Replication Protein A (RPA) is an abundant multi-domain heterotrimeric protein complex essential to nearly all DNA processing events inside eukaryotic cells. RPA is thus a critical component for replication, repair, and recombination pathways. The largest subunit, Rfa1, possesses four OB domains: DNA-binding domain-A (DBD-A), B (DBD-B), C (DBD-C), and F (DBD-F), which are connected by flexible linkers. The smallest subunit Rfa3 has a single OB-fold (DBD-E) and forms part of the trimerisation core (Tri-C) consisting of DBD-C of Rfa1, DBD-D of Rfa2, and DBD-E of Rfa3.

We produced recombinant full-length S. cerevisiae RPA heterotrimer complexes of Rfa1, Rfa2, and Rfa3 in bacteria (denoted as ScRPA). Recombinant ScRPA was purified to homogeneity as judged by SDS–PAGE and gel filtration analysis coupled with in-line multi-angle laser light scattering (SEC-MALS), suggesting intact complexes. We used a 100 nt polypyrimidine oligonucleotide to form a RPA-ssDNA complex containing multiple RPA molecules (dT100 and Supplementary Fig. 2a, b). Combining two datasets and several rounds of 2D and 3D classification we isolated a fraction of the particles that enabled a 3D reconstruction corresponding to the ScRPA Tri-C associated with ssDNA to a global resolution of 4.7 Å, a surprisingly high-resolution structure by cryoEM given the small size of the protein–nucleic acid complex (~55 kDa with ssDNA). Although full-length proteins were used to form the ScRPA-ssDNA complexes,, the winged-helix domain, as well as some of the N-terminus of Rfa2 were invisible. The reconstruction measures ~81 Å × ~58 Å × ~36 Å in dimensions and a model of the ScRPA Tri-C (based on homology models) can be fitted into the EM density map. Subsequently, the model was flexibly fitted using molecular dynamics flexible fitting (MDFF)32,33 and further refined using jelly-body refinement routines in Refmac534 within CCPEM35, and real-space refinement procedures in Phenix36. There are a number of yeast-specific insertions compared to the human or fungal structures, the most obvious being for DBD-D and DBD-E. The presence of ssDNA in the reconstruction is further supported by the observation that in the absence of ssDNA, RPA molecules do not assemble into dimers and trimers and the majority of the Tri-C particles were isolated from dimers and trimers. We were able to reconstruct the relatively small Tri-C stably bound to a 20-nt segment of the ssDNA to surprisingly high resolution given its low molecular mass (~55 kDa). Our studies suggest that DBD-A/DBD-B may be more dynamic than previously thought, whereas the trimerization core is more stable on ssDNA.

> MASETPRVDPTEISNVNAPVFRIIAQIKSQPTESQLILQSPTISSKNGSEVEMITLNNIRVSMNKTFEIDSWYEFVCRNNDDGELGFLILDAVLCKFKENEDLSLNGVVALQRLCKKYPEIY;> TNTRVNTLTPVTIKQILESKQDIQDGPFVSHNQELHHVCFVGVVRNITDHTANIFLTIEDGTGQIEVRKWSEDAAQQFEIGGYVKVFGALKEFGGKKNIQYAVIKPIDSFNEVLTHHLEVIKCHSIASGMMK;> KFIAQRITIARAQAENLGRSEKGDFFSVKAAISFLKVDNFAYPACSNENCNKKVLEQPDGTWRCEKCDTNNARPNWRYILTISIIDETNQLWLTLFDDQAKQLLGVDANTLMSLKEEDPNEFTKITQSIQMNEYDFRIRAREDTYNDQSRIRYTVANLHSLNYRAEADYLADELSKAL>[2x]REEGGVGSEEGVGKQCHPSLPPRCPSRSPSDQPWTHPDQSQLFADLSREELTTVMSFLTQQLGPDLVDAAQARPSDNCVFSVELQLPPKAAALAHLDRGSPPPAREALAIVFFGGQPQPNVTELVVGPLPQPSYMRDVTVERHGGPLPYYRRPVLLREYLDIDQMIFNRELPQAAGVLHHCCSYKQGGQKLLTMNSAPRGVQSGDRSTWFGIYYNITKGGPYLHPVGLELLVDHKALDPADWTVQKVFFQGRYYENLAQLEEQFEAGQVNVVVIPDDGTGGFWSL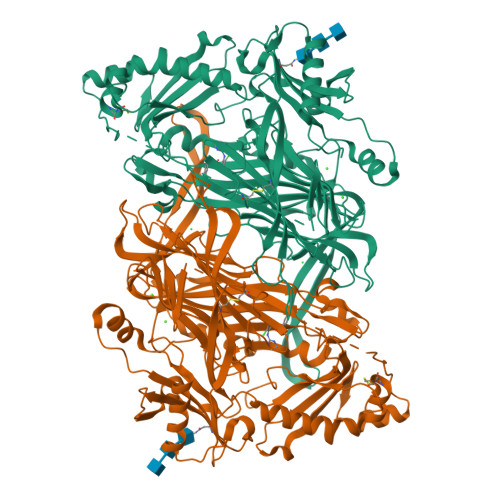KSQVPPGPTPPLQFHPQGPRFSVQGNRVASSLWTFSFGLGAFSGPRVFDVRFQGERLAYEISLQEAGAVYGGNTPAAMLTRYMDSGFGMGYFATPLIRGVDCPYLATYMDWHFVVESQTPKTLHDAFCVFEQNKGLPLRRHHSDFLSHYFGGVAQTVLVFRSVSTMLNYDYVWDMVFYPNGAIEVKLHATGYISSAFLFGAARRYGNQVGEHTLGPVHTHSAHYKVDLDVGGLENWVWAEDMAFVPTAIPWSPEHQIQRLQVTRKQLETEEQAAFPLGGASPRYLYLASKQSNKWGHPRGYRIQTVSFAGGPMPQNSPMERAFSWGRYQLAITQRKETEPSSSSVFNQNDPWTPTVDFSDFINNETIAGKDLVAWVTAGFLHIPHAEDIPNTVTVGNGVGFFLRPYNFFDQEPSMDSADSIYFREGQDAGSCEINPLACLPQAATCAPDLPVFSHGGYPEY> DVSGTVCLSALPPEATDTLNLIASDGPFPYSQDGVVFQNRESVLPTQSYGYYHEYTVITPGARTRGT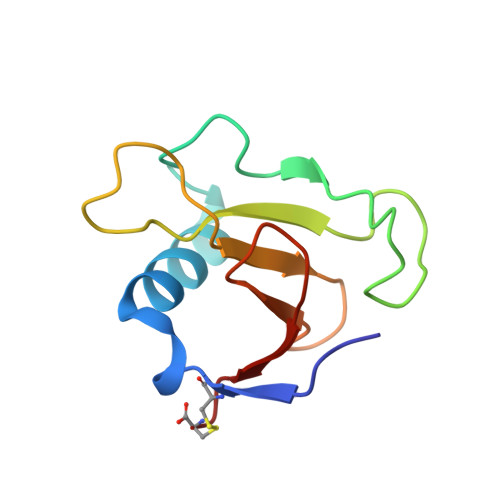RRIITGEAWQEDYYTGDHYATFSLIDQTC N-[(1S)-2-oxo-1-[3-(trifluoromethyl)phenyl]-2-({4-[4-(trifluoromethyl)phenyl]pyridin-3-yl}amino)ethyl]-4-[4-(trifluoromethyl)phenyl]pyridine-3-carboxamide | C34 H21 F9 N4 O2 | 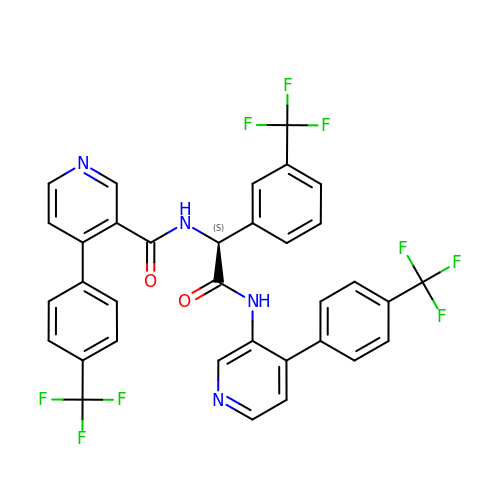BXBAJPGXWPVCNU-LJAQVGFWSA-N>[2x]GAMADRDRLRPPLDERSLRDQLIGAGSGWRQLDVVAQTGSTNADLLARAASGADIDGVVLIAEHQTAGRGRHGRGWAATARAQIILSVGVRVVDVPVQAWGWLSLAAGLAVLDSVAPLIAVP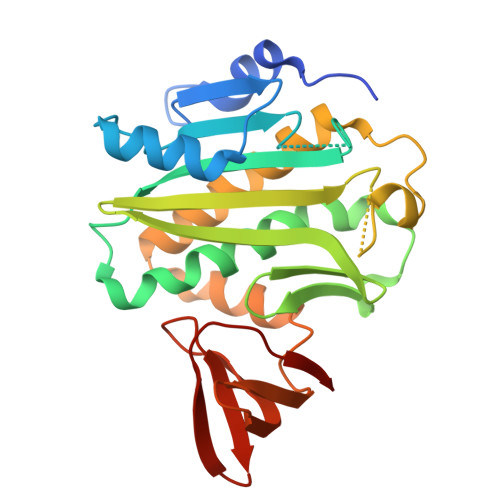PAETGLKWPNDVLARGGKLAGILAEVAQPFVVLGVGLNVTQAPEEVDPDATSLLDLGVAAPDRNRIASRLLRELEARIIQWRNANPQLAADYRARSLTIGSRVRVELPGGQDVVGIARDIDDQGRLCLDVGGRTVVVSAGDVVHLR>MGSSHHHHHHSSGLGVLPGGPLHMEEKLAVSLQEALQEGDTRALREVLEEIHPQDLLALWDELKGEHRYVVLTLLPKAKAAEVLSHLSPEEQAEYLKTLPPWRLREILEELSLDDLADALQAVRKEDPAYFQRLKDLLDPRTRAEVEALARYEEDEAGGLMTPEYVAVREGMTVEEVLRFLRRAAPDAETIYYIYVVDEKGRLKGVLSLRDLIVADPRTRVAEIMNPKVVYVRTDTDQEEVARLMADYDFTVLPVVDEEGRLVGIVTVDDVLDVLEAEATEDIHKLGAVDVP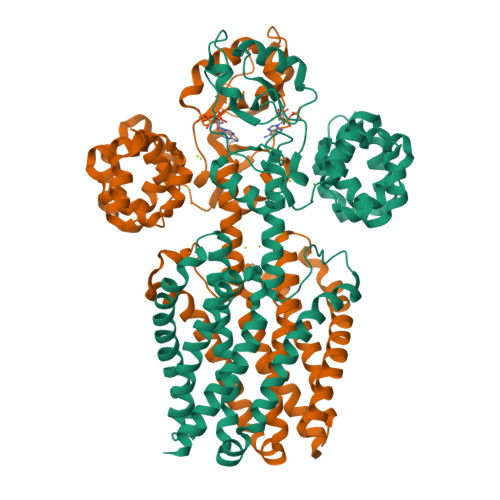DLVYSEAGPVALWLARVRWLVILILTGMVTSSILQGFESVLEAVTALAFYVPVLLGTGGNTGNQSATLIIRALATRDLDLRDWRRVFLKEMGVGLLLGLTLSFLLVGKVYWDGHPLLLPVVGVSLVLIVFFANLVGAMLPFLLRRLGVDPALVSNPLVATLSDVTGLLIYLSVARLLLEAV[2x]>SMDFKENPNLRDNWTDAEGYYRVNIGEVLDKRYNVYGYTGQGVFSNVVRARDNARANQEVAVKIIRNNELMQKTGLKELEFLKKLNDADPDDKFHCLRLLRHFYHKQHLCLVFEPLSMNLREVLKKYGKDVGLHIKAVRSYSQQLFLALKLLKRCNILHADIKPDNILVNESKTILKLCDFGSASHVADNDITPYLFSRFYRAPEIIIGKSYDYGIDMWSVGCTLYELYTGKILFPGKTNNHMLKLAMDLKGKMPNKMIRKGVFKDQHFDQNLNFMYIEVDKVTEREKVTVMSTINPTKDLLA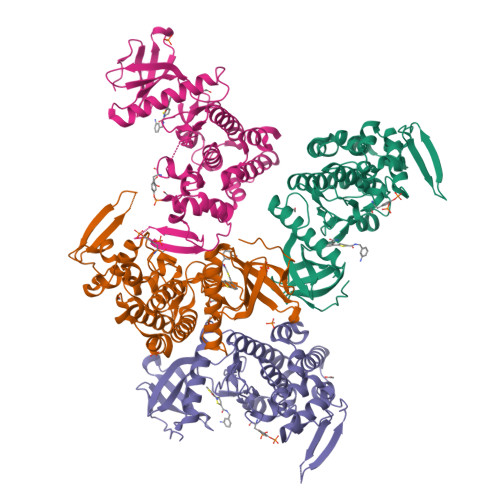DLIGCQRLPEDQRKKVHQLKDLLDQILMLDPAKRISINQALQHAFIQE[4x]Crocagins (1 and 2)24 are very small, intriguing RiPPs that possess a tetracyclic ring system, which consists of a pyrroloindoline fused to a tetrahydropyrimidinone moiety. Here we use in vitro experiments to demonstrate that three proteins, CgnB, CgnC and CgnE, are sufficient for the production of the hallmark tetracyclic crocagin core from the precursor peptide CgnA. We further show that the hydrolase CgnD liberates the crocagin core scaffold, which is subsequently N-methylated by CgnL. The crystal structures of the homologues CgnB and CgnE reveal them to be the founding members of a peptide-binding protein family and allow us to rationalize their distinct functions.

Based on sequence alignments, CgnL, named ‘MT’ in the original crocagin publication, was the likely candidate. Indeed, incubation of 4a and 4b with CgnL and S-adenosylmethionine led to the formation of 5a ([M]+ calculated, 509.2395; observed, 509.2391; Δ = –0.8 ppm) and the –2 Da 5b ([M]+ calculated, 507.2238; observed, 507.2239; Δ = 0.2 ppm; Fig. 4c and Supplementary Fig. 21). The mass increase of +14 Da suggested methylation and thus the production of des-carbamoyl 1 and 2. The crystal structure of CgnL in complex with S-adenosylhomocysteine was determined to a resolution of 1.96 Å and appeared monomeric, which was consistent with the closest structural homologues of CgnL identified in a Dali search. The overall shape of CgnL was typical for class I S-adenosylmethionine-dependent methyltransferases with a Rossman fold. The electron density for S-adenosylhomocysteine was unambiguous as expected for a well-coordinated ligand.

>GAMGGGGYHLFNELAHSYDLHTPPENFQHDHAFVLEEARSLGTPCRLLDVGCGTGALLEKARNAGILATGIDASPKMVELAQARVGQEAVTLRRMEEIDEEGAYDLVVSLCWTIHYSAGRAGLLDVLKRIHRALRPGGRGIIQIAHAAHAPKRTLESRIPGPNGEPDDVVMLFRFRPAPTEEPSMHAEYVYACKSLNELLYENHLLSMTDAHAFAACAREAGFAQVTVYDSSKRAPFSAAPNPLVCVEKAHDVGR[4x]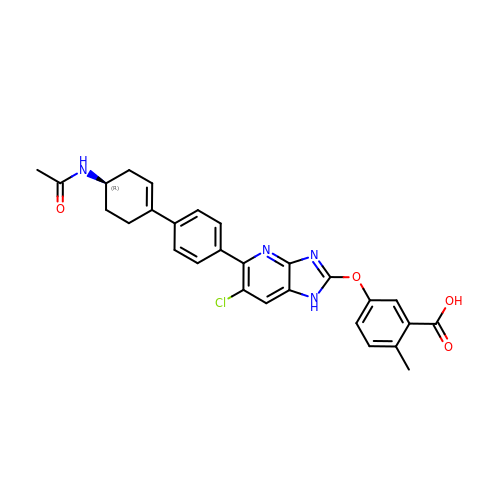5-({5-[(4'R)-4'-acetamido-2',3',4',5'-tetrahydro[1,1'-biphenyl]-4-yl]-6-chloro-1H-imidazo[4,5-b]pyridin-2-yl}oxy)-2-methylbenzoic acid | C28 H25 Cl N4 O4 | DYYYOJWTTPYOIK-FQEVSTJZSA-N>MTEAQAIAKQLGGVKPDDEWLQAEIARLKGKSIVPLQQVKTLHDWLDGKRKARKSCRVVGESRTGKTVACDAYRYRHKPQQEAGRPPTVPVVYIRPHQKCGPKDLFKKITEYLKYRVTKGTVSDFRDRTIEVLKGCGVEMLIIDEADRLKPETFADVRDIAEDLGIAVVLVGTDRLDAVIKRDEQVLERFRAHLRFGKLSGEDFKNTVEMWEQMVLKLPVSSNLKSKEMLRILTSA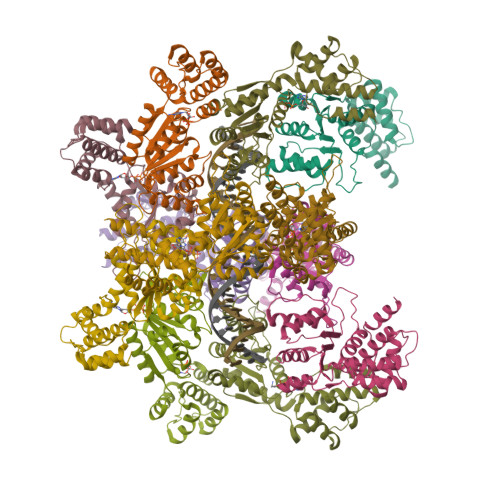TEGYIGRLDEILREAAIRSLSRGLKKIDKAVLQEVAKEYK[12x]>LKLCSPEEFTRLCREKTQEIYPIKEANGRTRKALIICNTEFKHLSLRYGANFDIIGMKGLLEDLGYDVVVKEELTAEGMESEMKDFAALSEHQTSDSTFLVLMSHGTLHGICGTMHSEKTPDVLQYDTIYQIFNNCHCPGLRDKPKVIIVQAARGGNSGEMWIRESSKPQLCRGVDLPRNMEAD[2x];>[3x]KLSHVEKDFIAFYSTTPHHLSYRDKTGGSYFITRLISCFRKHACSCHLFDIFLKVQQSFEKASIHSQMPTIDRATLTRYFYLFPGN;> TLKLCSPEEFTRLCREKTQEIYPIKEANGRTRKALIICNTEFKHLSLRYGANFDIIGMKGLLEDLGYDVVVKEELTAEGMESEMKDFAALSEHQTSDSTFLVLMSHGTLHGICGTMHSEKTPDVLQYDTIYQIFNNCHCPGLRDKPKVIIVQAARGGNSGEMWIRESSKPQLCRGVDLPRNMEAD;> VKLSHVEKDFIAFYSTTPHHLSYRDKTGGSYFITRLISCFRKHACSCHLFD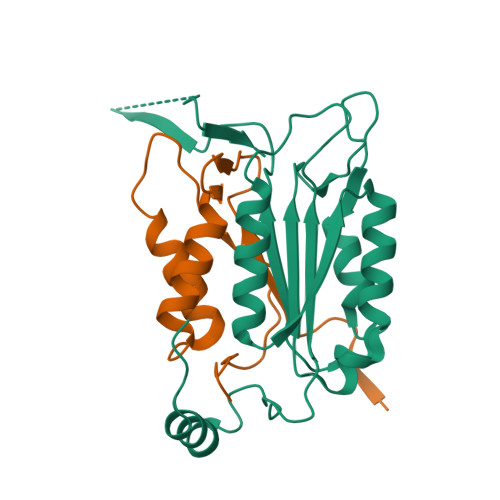IFLKVQQSFEKASIHSQMPTIDRATLTRYFYLFPGN;> TLKLCSPEEFTRLCREKTQEIYPIKEANGRTRKALIICNTEFKHLSLRYGANFDIIGMKGLLEDLGYDVVVKEELTAEGMESEMKDFAALSEHQTSDSTFLVLMSHGTLHGICGTMHSEKTPDVLQYDTIYQIFNNCHCPGLRDKPKVIIVQAA>ASMTGGQQMGAPITAYAQQTRGLLGCIITSLTGRDKNQVEGEVQIVSTATQTFLATCINGVCWTVYHGAGTRTIASPKGPVIQMYTNVDQDLVGWPAPQGSRSLTPCTCGSSDLYLVTRHADVIPVRRRGDSRGSLLSPRPISYLKGSSGGPLL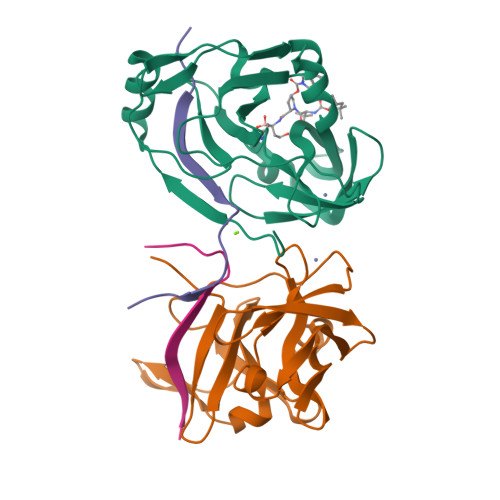CPAGHAVGLFRAAVCTRGVAKAVDFIPVENLETTMRGSHHHHHH[2x];>KKGSVVIVGRIVLSGKPAIIPKK[2x]> 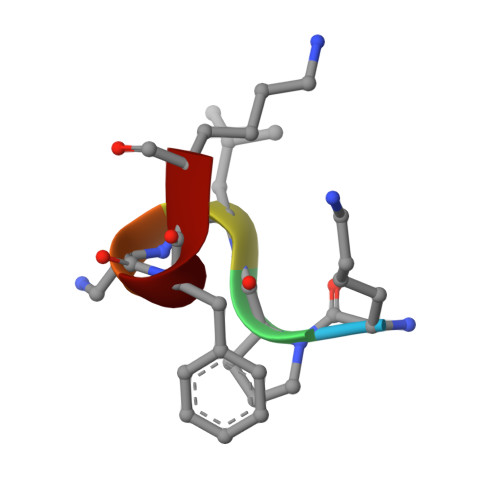KPLAFK> VLEEDREPDFIEV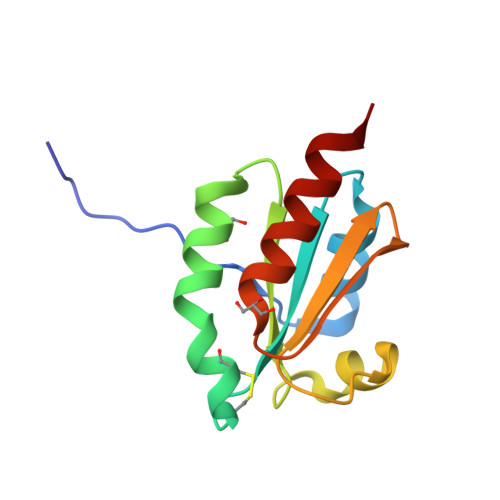NSLEEFDEIMSMDILTVAWFWAEDCGPCKLIEEPLRKMAEEFPNVVFARVDADKNPEIVKKLNIKSLPTAVIARSGEYLGDVVGARPDLLREKVENILKNLE>[4x]MDNQKGRISI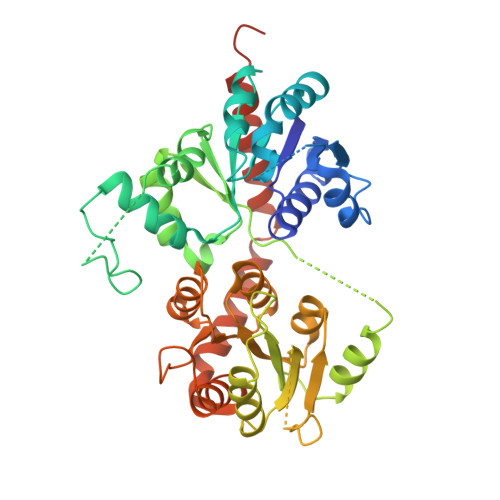ALLPFLAHGHISPFFELAKQLAKRNCNVFLCSTPINLSSIKDKDSSASIKLVELHLPSSPDLPPHYHTTNGLPSHLMLPLRNAFETAGPTFSEILKTLNPDLLIYDFNPSWAPEIASSHNIPAVYFLTTAAASSSIGLHAFKNPGEKYPFPDFYDNSNIIPEPPSADNMKLLHDFIACFERSCDIILIKSFRELEGKYIDLLSTLSDKTLVPVGPLVQDPMGHNEDPKTEQIINWLDKRAESTVVFVCFGSEYFLSNEELEEVAIGLEISTVNFIWAVRLIEGEKKGILPEGFVQRVGDRGLVVEGWAPQARILGHSSTGGFVSHCGWSSIAESMKFGVPVIAMARHLDQPLNGKLAAEVGVGMEVVRDENGKYKREGIAEVIRKVVVEKSGEVIRRKARELSEKMKEKGEQEIDRAVEELVQICKKKKDEQENLYFQGHHHHHH>[2x]GSHMASMTGGQQMGRGSEDSLTKQPEEVFDVLEKLGEGS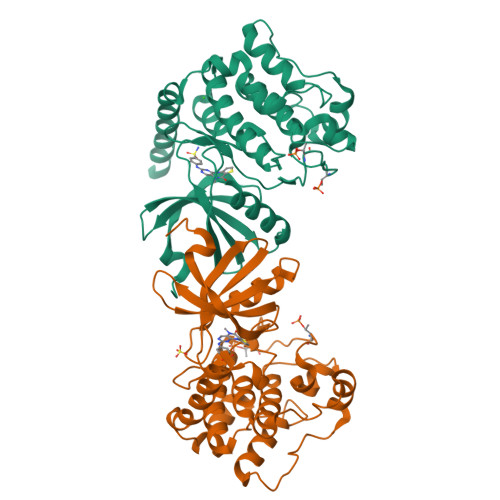YGSVFKAIHKESGQVVAIKQVPVESDLQEIIKEISIMQQCDSPYVVKYYGSYFKNTDLWIVMEYCGAGSVSDIIRLRNKTLIEDEIATILKSTLKGLEYLHFMRKIHRDIKAGNILLNTEGHAKLADFGVAGQLTDTMAKRNTVIGTPFWMAPEVIQEIGYNCVADIWSLGITSIEMAEGKPPYADIHPMRAIFMIPTNPPPTFRKPELWSDDFTDFVKKCLVKNPEQRATATQLLQHPFIKNAKPVSILRDLITEAMEIKAKRHEEQQRELEEEE> VRSRNGGATKIVREHYLRSDIPCLSRSCTKCPQIVVPDAQNELPKFILSDSPLELSAPIGKHYVVLDTNVVLQAIDLLENPNCFFDVIVPQIVLDEVRNKSYPVYTRLRTLCRDSDDHKRFIVFHNEFSEHTFVERLPNETINDRNDRAIRKTCQWYSEHLKPYDINVVLVTNDRLNREAATKEVESNIITKSLVQYIELLPNADDIRDSIPQMDSFDKDLERDTFSDFTFPEYYSTARVMGGLKNGVLYQGNIQISEYNFLEGSVSLPRFSKPVLIVGQKNLNRAFNGDQVIVELLPQSEWKAPSSIVLDSEHFDVNDNPDIEAGDDDDNNESSSNTTVISDKQRRLLAKDAMIAQRSKKIQPTAKVVYIQRRSWRQYVGQLAPSSVDPQSSSTQNVFVILMDKCLPKVRIRTRRAAELLDKRIVISIDSWPTTHKYPLGHFVRDLGTIESAQAETEALLLEHDVEYRPFSKKVLECLPAEGHDWKAPTKLDDPEAVSKDPLLTKRKDLRDKLICSIDPPGCVDINDALHAKKLPNGNWEVGVHIADVTHFVKPGTALDAEGAARGTSVYLVDKRIDMLPMLLGTDLCSLKPYVDRFAFSVIWELDDSANIVNVNFMKSVIRSREAFSYEQAQLR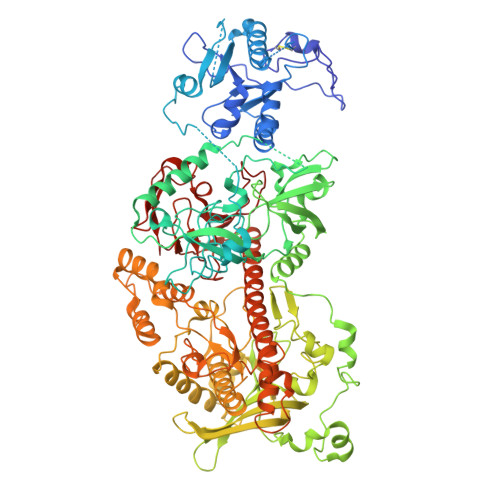IDDKTQNDELTMGMRALLKLSVKLKQKRLEAGALNLASPEVKVHMDSETSDPNEVEIKKLLATNSLVEEFMLLANISVARKIYDAFPQTAMLRRHAAPPSTNFEILNEMLNTRKNMSISLESSKALADSLDRCVDPEDPYFNTLVRIMSTRCMMAAQYFYSGAYSYPDFRHYGLAVDIYTHFTSPIRRYCDVVAHRQLAGAIGYEPLSLTHRDKNKMDMICRNINRKHRNAQFAGRASIEYYVGQVMRNNESTETGYVIKVFNNGIVVLVPKFGVEGLIRLDNLTEDPNSAAFDEVEYKLTFVPTNSDKPRDVYVFDKVEVQVRSVMDPITSKRKAELLLK Puromycin and the Streptomyces alboniger-derived puromycin N-acetyltransferase (PAC) enzyme form a commonly used system for selecting stably transfected cultured cells. The crystal structure of PAC has been solved using X-ray crystallography, revealing it to be a member of the GCN5-related N-acetyltransferase (GNAT) family of acetyltransferases. PAC adopts a fold consistent with the GCN5-related N-acetyltransferase (GNAT) family, consisting of a seven-stranded β-sheet interspersed with four α-helices. PAC displays the typical structural hallmarks of this family which includes a cleft in the middle of the sheet between the parallel strands 4 and 5 that facilitates AcCoA binding.

In the absence of cofactor or substrate, PAC was highly unstable and readily precipitated. Addition of either acetyl-CoA (AcCoA) or puromycin to PAC in solution greatly improved its thermal stability, with a 12 °C increase in melting temperature. The addition of AcCoA enabled crystallisation of PAC and the determination of its three-dimensional structure using X-ray crystallography. AcCoA binding is primarily through a “P-loop” formed by a conserved Q–X–X–G–X–G motif in the loop after β-strand 4, which allows the coordination of the pyrophosphate moiety of the CoA by the protein backbone. The poor initial electron density around the adenine moiety of the CoA made its unambiguous placement difficult and the adenine moiety has been modelled in both orientations.

>MGSTEYKPTVRLATRDDVPRAVRTLAAAFADYPATRHTVDPDRHIERVTELQELFLTRVGLDIGKVWVADDGAAVAVWTTPESVEAGAVFAEIGPRMAELSGSRLAAQQQMEGLLAPHRPKEPAWFLATVGVSPDHQGKGLGSAVVLPGVEAAERAGVPAFLETSAPRNLPFYERLGFTVTADVEVPEGPRTWCMTRKPGASHHHHHH[6x]>QEVEFDIPPQALGSALQEFGRQADIQVLYRPEEVRNKRSSAIKGKLEPNQAITELLRGTGASVDFQGNAITISVAEAADSSVDLGATMITSNQLGTITEDSGSYTPGTIATATRLVLTPRETPQSITVVTRQNMDDFGLNNIDDVMRHTPGITVSAYDTDRNNYYARGFSINNFQYDGIPSTARNVGYSAGNTLSDMAIYDRVEVLKGATGLLTGAGSLGATINLIRKKPTHEFKGHVELGAGSWDNYRSELDVSGPLTESGNVRGRAVAAYQDKHSFMDHYERKTSVYYGILEFDLNPDTMLTVGADYQDNDPKGSGWSGSFPLFDSQGNRNDVSRSFNNGAKWSSWEQYTRTVFANLEHNFANGWVGKVQLDHKINGYHAPLGAIMGDWPAPDNSAKIVAQKYTGETKSNSLDIYLTGPFQFLGREHELVVGTSASFSHWEGKSYWNLRNYDNTTDDFINWDGDIGKPDWGTPSQYIDDKTRQLGSYMTARFNVTDDLNLFLGGRVVDYRVTGLNPTIRESGRFIPYVGAVYDLNDTYSVYASYTDIFMPQDSWYRDSSNKLLEPDEGQNYEIGIKGEYLDGRLNTSLAYFEIHEENRAEEDALYNSKPTNPAITYAYKGIKAKTKGYEAEISGELAPGWQVQAGYTHKIIRDDSGKKVSTWEPQDQLSLYTSYKFKGALDKLTVGGGARWQGKSWQMVYNNPRSRWEKFSQEDYWLVDLMARYQITDKLSASVNVNNVFDKTYYTNIGFYTSASYGDPRNLM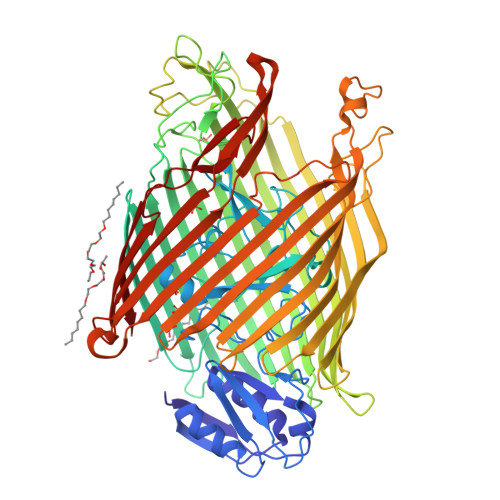FSTRWDF[2x];> SKGKSSGKKS> MLEEDKIKGMFNPKIWDKTFQDGLKKEIEDSQPYNWGTIHELVNDDLLRAVRKEIETEIHFTKKETDIYRVNQSGDLANLSGLDWDDLSRLPNLFKLRQILYSKQYRDFFGYVTKAGKLSGSKTDMSINTYTKGCHLLTHDDVIGSRRISFILYLPDPDRKWKSHYGGGLRLFPSILPNVPHSDPSAKLVPQFNQIAFFKVLPGFSFHDVEEVKVDKHRLSIQGWYHIPQVGEEGYIPGEEEAWVRNNTSTLAQIESNVLEDFEFPKDERNILSFHEVKHFEKMLKGDAGAKTDNTPKESMTSVISDSVKLSEAEFTYLSQYISPEHLSSKGIEKLQ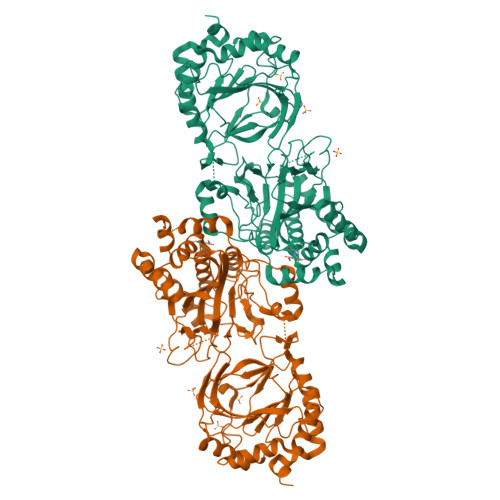KQFVENSSLQIESFLNDDKSELLKKVIKQKELEQECPYHSKDVKAPWKTAIPPHKARYLYIDGKEYRNFQTEADILEALNNNDLPNFQFTKDAIKIISDASGNSRENNFDAELALIDLAVFHKSTIFKKYLALLTSLCPVSEQILIRRFRPGMDFTLATKCRFNELLKSNPDIIDAVLEGTLCLTPSAGWESGELGGYELYMMDDDEDNKQYLKEDVEDASVYRADDSGDSVLINDPPAWNTFNLVLRDESVLEFVKYVSWSAKSSRWDVKMKWDVKSCDEDGQEDEALEHHHHHH> RHSGS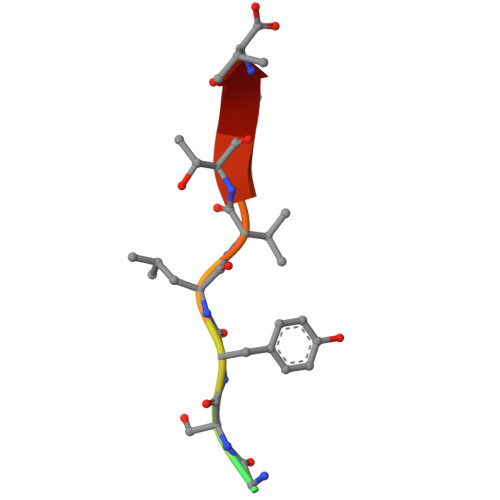YLVTSV>NKTHQVEHESEQSDFQDIRFGLNSVKLPKAQPAAATRITVENGTDKLVNYKSSPQQLFLAKNALKDKLQGEFDKFLSDAKAFPALTADLQEWVDQQLFNPNQSFFDLSAPRSNFTLSSDKKASLDFIFRFTNFTESVQLLKLPEGVSVVVDSKQSFDYYVNASAQKLLVLPLSLPDYTLGLNYMFDHITLNGKVVNKFSFNPFKTNLNLAFSNVYNGVDVFEAQKNLVGKGKYLNTHVKAEDVKKDVNANIKNQFDIAKIIAELMGKALKEFGNQQEGQPLSFLKVMDKVKEDFEKLFNLVRPGLGKFVKDLIQSSSQAENKITVYKLIFDNKKTILNLLKELSIPELNSSLGLVDVLFDGITDSDGLYERLQSFKDLIVPAVKTNEKTAALSPLIEELLTQKDTYVFDLIQKHKGILTNLLKNFLADFQKSTPFMADQVAIFTELFDNEGAFDLFGEADFVDKIAELFLTKRTVKNGEKIETKDSLLVTSLKSLLGEKVAALGDLLDSYIFKNELLNRSVEVAKAEAKDTKGATDYKKEQAKALKKLFKHIGENTLSKTNLDKITLKEVKNTENVELEETETTLKVKKLDVEYKVELGNFEIKNGLIKAMLEFLPDTKDLETTLDKLLFKGESYKAMKDKYIKEGFPGYGWAKGVVPGAFESIENTFKSAIDKTKSIRDLFGDMLFGNDLSSVKETDSFITLGGSFDIKYGGENLNVLPAYYSLINSEIGYQIIGVDTTIDATKVKVELKNKEYKGKSPAINGQVKLSQSFFNVWTNMFDSITKQIFQKKYEFKDNIQVFARNEDNTSRLELDISDPEQRVIPFAFVDGFGIQLKAVDKNITKEAGNTEPKSPVIQLYEA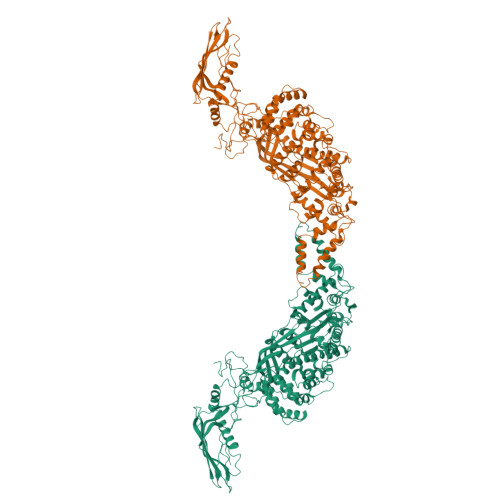LNKEKDQKQQSKQSPKQLDTKTQLGYLLKLGDNWSKDDYKSLIDDTIINNNYLEASFNSKITVDRLGIPIDLWLFKIWPKFNLEIPMQGSLQLYSSSVIFPYGIYDTSVQDAAKIVKRLNFTDMGFKLNDPKPNFWFVGFKHHHHH[2x]>MLSNELRQTLQKGLHD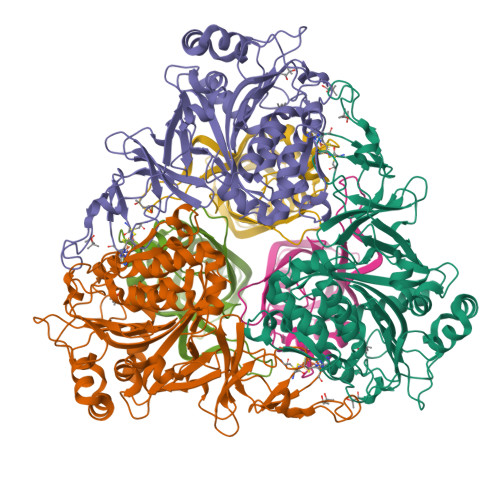VNSDWTVPAAIINDPEVHDVERERIFGHAWVFLAHESEIPERGDYVVRYISEDQFIVCRDEGGEIRGHLNACRHRGMQVCRAEMGNTSHFRCPYHGWTYSNTGSLVGVPAGKDAYGNQLKKSDWNLRPMPNLASYKGLIFGSLDPHADSLEDYLGDLKFYLDIVLDRSDAGLQVVGAPQRWVIDANWKLGADNFVGDAYHTMMTHRSMVELGLAPPDPQFALYGEHIHTGHGHGLGIIGPPPGMPLPEFMGLPENIVEELERRLTPEQVEIFRPTAFIHGTVFPNLSIGNFLMGKDHLSAPTAFLTLRLWHPLGPDKMEVMSFFLVEKDAPDWFKDESYKSYLRTFGISGGFEQDDAENWRSITRVMGGQFAKTGELNYQMGRGVLEPDPNWTGPGEAYPLDYAEANQRNFLEYWMQLMLAESPLRDGNSNGSGTADASTPAAAKSKSPAKAEA[3x];>MNTQTRVSDTTVREITEWLYMEAELLDAGKYREWLALVTEDLSYVVPIRVTREREAVTDVVEGMTHMDDDADSMEMRVLRLETEYAWAEDPPSRSRHFVTNVRVATGDSEDEFKVTSNLLLYRTRGDVATYDVLSGERTDVLRRAGDSFLMAKRVVLLDQTTIMTHNLALIM[3x]URIDINE-DIPHOSPHATE-3(N-ACETYLGLUCOSAMINYL)BUTYRIC 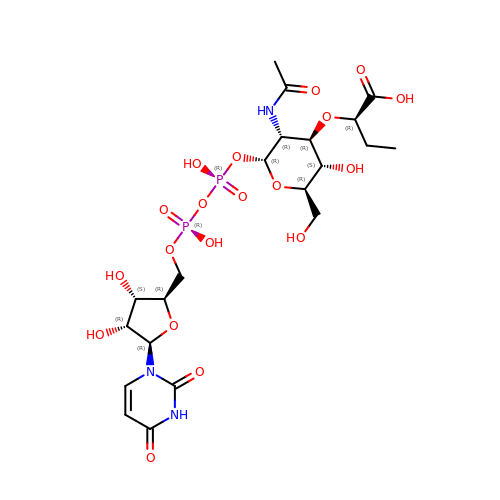ACID | C21 H33 N3 O19 P2 | DFCARJAECCPPGB-LHYXAPFASA-N Using soluble chitin derivatives as oligoglycosyl donor and oligosaccharides derived from chitin and β-1,3-glucan as acceptors, A. fumigatus Crh enzymes act as transglycosylases for formation of chitin–chitin and chitin–glucan crosslinks both in vitro and in vivo. AfCrh5 adopts the GH16 family β-jelly-roll fold composed of two stacked seven-stranded β-sheets with a convex and a concave face. AfCrh5 shares the general EXDXE active site motif present in most GH16 family enzymes in which the first glutamate, the middle aspartate and the last glutamate act as the catalytic nucleophile, the auxiliary residue, and the general acid/base, respectively. In AfCrh5, Glu119 and Glu123 are predicted to act as the nucleophile and the general acid/base, respectively.

To address these questions, we determined the apo crystal structure of AfCrh5 and its crystal structure in complex with chitooligosaccharides. Apo crystals were obtained using ammonium sulphate as a precipitant and diffracted to 2.25 Å. The apo and the complexed structure were solved by molecular replacement and refined to 0.23 and 0.24 R/Rfree values, respectively. Both crystals belong to the same orthorhombic space group with two independent molecules in the asymmetric unit (AU). No conformational changes were observed between the apo and the complexed AfCrh5 structures or between the AU molecules with overall root-mean-square deviation (RMSD) values of 0.20 and 0.25 Å for 213 Cα atoms, respectively. Finally, a truncated form of AfCrh5 (residues 22–275, excluding the signal peptide, the Ser/Thr-rich region and GPI-anchor sequences) was expressed as a fusion protein featuring an N-terminal PreScission cleavable GST-tag followed by a His-tag.

>[2x]WSKCNPLEKTCPPNKGLAASTYTADFTSASALDQWEVTAGKVPVGPQGAEFTVAKQGDAPTIDTDFYFFFGKAEVVMKAAPGTGVVSSIVLESDDLDEVDWEVLGGDTTQVQTNYFGKGDTTTYDRGTYVPVATPQETFHTYTIDWTKDAVTWSIDGAVVRTLTYNDAKGGTRFPQTPMRLRLGSWAGGDPSNPKGTIEWAGGLTDYSAGPYTMYVKSVRIENANPAESYTYSDNSGSWQSIKFD> METVISSDSSPAVENEHPQETPESNNSVYTSFMKSHRCYDLIPTSSKLVVFDTSLQVKKAFF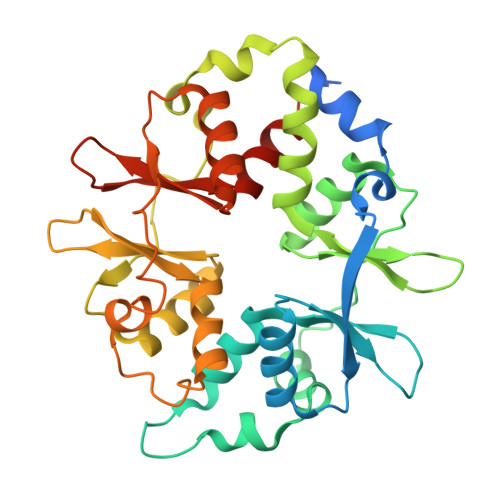ALVTNGVRAAPLWDSKKQSFVGMLTITDFINILHRYYKSALVQIYELEEHKIETWREVYLQDSFKPLVCISPNASLFDAVSSLIRNKIHRLPVIDPESGNTLYILTHKRILKFLKLFITEFPKPEFMSKSLEELQIGTYANIAMVRTTTPVYVALGIFVQHRVSALPVVDEKGRVVDIYSKFDVINLAAEKTYNNLDVSVTKALQHRSHYFEGVLKCYLHETLETIINRLVEAEVHRLVVVDENDVVKGIVSLSDILQALVLTGGEKKP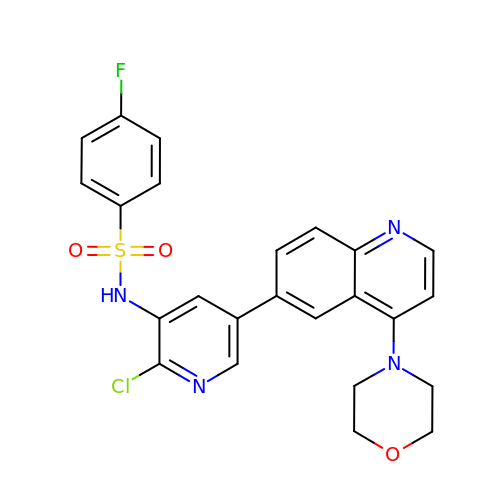N-{2-chloro-5-[4-(morpholin-4-yl)quinolin-6-yl]pyridin-3-yl}-4-fluorobenzenesulfonamide | C24 H20 Cl F N4 O3 S | RTARVPHTCQRSDW-UHFFFAOYSA-N> PISPIETVPVKLKPGMDGPKVKQWPLTEEKIKALVEICTEMEKEGKISKIGPENPYNTPVFAIKKKDSTKWRKLVDFRELNKRTQDFWEVQLGIPHPAGLKKKKSVTVLDVGDAYFSVPLDEDFRKYTAFTIPSINNETPGIRYQYNVLPQGWKGSPAIFQSSMTKILEPFRKQNPDIVICQYMDDLYVGSDLEIGQHRTKIEELRQHLLRWGLTTPDKKHQKEPPFLWMGYELHPDKWTVQPIVLPEKDSWTVNDIQKLVGKLNWASQIYPGIKVRQLCKLLRGTKALTEVIPLTEEAELELAENREILKEPVHGVYYDPSKDLIAEIQKQGQGQWTYQIYQEPFKNLKTGKYARMRGAHTNDVKQLTEAVQKITTESIVI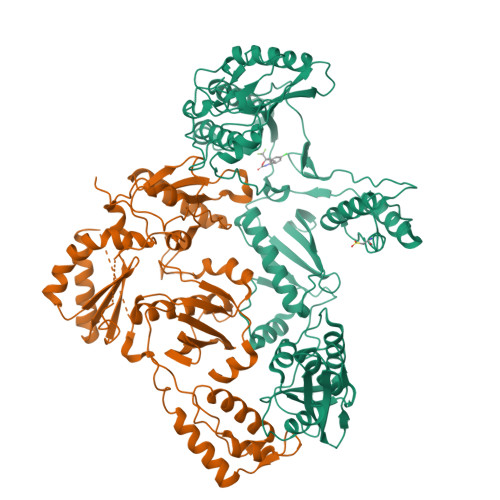WGKTPKFKLPIQKETWETWWTEYWQATWIPEWEFVNTPPLVKLWYQLEKEPIVGAETFYVDGAANRETKLGKAGYVTNRGRQKVVTLTDTTNQKTELQAIYLALQDSGLEVNIVTDSQYALGIIQAQPDQSESELVNQIIEQLIKKEKVYLAWVPAHKGIGGNEQVDKLVSAGIRKVL;> PISPIETVPVKLKPGMDGPKVKQWPLTEEKIKALVEICTEMEKEGKISKIGPENPYNTPVFAIKKKDSTKWRKLVDFRELNKRTQDFWEVQLGIPHPAGLKKKKSVTVLDVGDAYFSVPLDEDFRKYTAFTIPSINNETPGIRYQYNVLPQGWKGSPAIFQSSMTKILEPFRKQNPDIVICQYMDDLYVGSDLEIGQHRTKIEELRQHLLRWGLTTPDKKHQKEPPFLWMGYELHPDKWTVQPIVLPEKDSWTVNDIQKLVGKLNWASQIYPGIKVRQLCKLLRGTKALTEVIPLTEEAELELAENREILKEPVHGVYYDPSKDLIAEIQKQGQGQWTYQIYQEPFKNLKTGKYARMRGAHTNDVKQLTEAVQKITTESIVIWGKTPKFKLPIQKETWETWWTEYWQATWIPEWEFVNTPPLVKLWYQLEKEPIVGAETF The V/A ATPase from the thermophilic eubacterium Thermus thermophilus (Tth) is one of the best characterized rotary ATPases. The a-subunit is connected to the A3B3 stator in the V1 domain by two peripheral EG stalks which form a peripheral stator apparatus (A3B3E2G2a1). In addition, the dodecamer c ring composed of two transmembrane α-helices, the d-subunit and the DF shaft constitute the central rotor complex (D1F1d1c12), which rotates relative to the surrounding stator apparatus. The proton motive force generated by respiratory complexes drives proton translocation through a proton pathway made up of both the a-subunit and the c12 ring.

After refinements, 57.9 % of the particles corresponded to state1 and gave maps at a resolution of 5.0 Å, higher than those of state2 at 6.7 Å resolution and state3 at 7.5 Å, containing 15.2% and 6.3% of the particles, respectively. Local resolution analysis by Resmap22 for state1 showed a range of resolution from ~ 4 Å in the V1 region to ~ 5 Å in the Vo domain, indicating conformational heterogeneity within the complex. Local resolution of the hydrophobic region, especially of the c12 ring, was limited to ~ 6 Å due to conformational heterogeneity even within the most populated state1 structure. In order to improve resolution of the Vo domain, we employed the focused classification by using signal subtraction of hydrophilic region for state1, as described in Supplementary Figure 3. The improved map of state1 at 5.0 Å resolution allowed us to build a model of the whole complex. The inclined α-helices a-TM7 and a-TM8 are intimately associated with the c12 ring composed of 12 c-subunits, each with two transmembrane α-helices joined by a short loop on the cytoplasmic side. The tilted a-TM7 contains the conserved R563, corresponding to R735 in the yeast enzyme, which together with E63 in the c-subunit forms an essential feature of proton translocation. The density for a-TM7, where the R563 is located, is in close proximity to the center of an outer helix of the c-subunit. The cytoplasmic cavity provides direct access to the hydrophilic residues on a-TM7, reaching the Arg-Glu pair between a-TM7 and the outer helix of c-subunit, suggesting that this cavity corresponds to the cytoplasmic half channel. The periplasmic cavity in the center of micelle shell faces the helix bundle composed of a-TM1, a-TM2, and a-TM3, including a line of hydrophilic residues, and connects to the aqueous hole giving an access to the inclined helices.

>[3x]MIQGVIQKIAGPAVIAKGMLGARMYDICKVGEEGLVGEIIRLDGDTAFVQVYEDTSGLKVGEPVVSTGLPLAVELGPGMLNGIYDGIQRPLERIREKTGIYITRGVVVHALDREKKWAWTPMVKPGDEVRGGMVLGTVPEFGFTHKILVPPDVRGRVKEVKPAGEYTVEEPVVVLEDGTELKMYHTWPVRRARPVQRKLDPNTPFLTGMRILDVLFPVAMGGTAAIPGPFGSGKTVTQQSLAKWSNADVVVYVGCGERGNEMTDVLVEFPELTDPKTGGPLMHRTVLIANTSNMPVAAREASIYVGVTIAEYFRDQGFSVALMADSTSRWAEALREISSRLEEMPAEEGYPPYLAARLAAFYERAGKVITLGGEEGAVTIVGAVSPPGGDMSEPVTQSTLRIVGAFWRLDASLAFRRHFPAINWNGSYSLFTSALDPWYRENVAEDYPELRDAISELLQREAGLQEIVQLVGPDALQDAERLVIEVGRIIREDFLQQNAYHEVDAYCSMKKAYGIMKMILAFYKEAEAAIKRGVSIDEILQLPVLERIGRARYVSEEEFPAYFEEAMKEIQGAFKALA;>MDLLKKEYTGITYISGPLLFVENAKDLAYGAIVDIKDGTGRVRGGQVIEVSEEYAVIQVFEETTGLDLATTSVSLVEDVARLGVSKEMLGRRFNGIGKPIDGLPPITPEKRLPITGLPLNPVARRKPEQFIQTGISTIDVMNTLVRGQKLPIFSGSGLPANEIAAQIARQATVRPDLSGEGEKEEPFAVVFAAMGITQRELSYFIQEFERTGALSRSVLFLNKADDPTIERILTPRMALTVAEYLAFEHDYHVLVILTDMTNYCEALREIGAAREEIPGRRGYPGYMYTDLATIYERAGVVEGKKGSVTQIPILSMPDDDRTHPIPDLTGYITEGQIQLSRELHRKGIYPPIDPLPSLSRLMNNGVGKGKTREDHKQVSDQLYSAYANGVDIRKLVAIIGEDALTENDRRYLQFADAFERFFINQGQQNRSIEESLQIAWALLSMLPQGELKRISKDHIGKYYGQKLEEIWGAPQALD[3x];> MSQVSPTRMNLLQRRGQLRLAQKGVDLLKKKRDALVAEFFGLVREAMEARKALDQAAKEAYAALLLAQAFDGPEVVAGAALGVPPLEGVEAEVENVWGSKVPRLKATFPDGALLSPVGTPAYTLEASRAFRRYAEALIRVANTETRLKKIGEEIKKTTRRVNALEQVVIPGIRAQIRFIQQVLEQREREDTFRLKRIKGKIEAREAEEEGGRPNPQVEIGAGL;> MAVIADPETAQGFRLAGLEGYGASSAEEAQSLLETLVERGGYALVAVDEALLPDPERAVERLMRGRDLPVLLPIAGLKEAFQGHDVEGYMRELVRKTIGFDIKL;>MTGGLVLNAISRAGGAMGGLGLIKSLAEKEKQLLERLEAAKKEAEERVKRAEAEAKALLEEAEAKAKALEAQYRERERAETEALLARYRERAEAEAKAVREKAMARLDEAVALVLKEVLP[2x];>[2x]MSKLEAILSQEVEAEIQALLQEAEAKAEAVKREAEEKAKALLQARERALEAQYRAALRRAESAGELLVATARTQARGEVLEEVRRRVREALEALPQKPEWPEVVRKLALEALEALPGAKALVANPEDLPHLEAMARERGVELQAEPALRLGVRAVGAEGKTQVENSLLARMDRAWDAMSSKVAQALWG;> MADDFAYLNARVRVRRGTLLKESFFQEALDLSFADFLRLLSETVYGGELAGQGLPDVDRAVLRTQAKLVGDLPRLVTGEAREAVRLLLLRNDLHNLQALLRAKATGRPFEEVLLLPGTLREEVWRQAYEAQDPAGMAQVLAVPGHPLARALRAVLRETQDLARVEALLAKRFFEDVAKAAKGLDQPALRDYLALEVDAENLRTAFKLQGSGLAPDAFFLKGGRFVDRVRFARLMEGDYAVLDELSGTPFSGLSGVRDLKALERGLRCVLLKEAKKGVQDPLGVGLVLAYVKEREWEAVRLRLLARRAYFGLPRAQVEEEVVCP;> MIAPMEKLVLAGPKGRAKELLQSLQQAGVVHLETLRPEALSAYQLSPEERAELRRWEAVSAGAEHTLSLLGLEAEPARPFPEGLEAAEKALSPIQAHAEGLTRQKQELEEELALAQAYLEPLERLAALAHGLDKSPFLRVIPFLLTEKELPLVEEALRKALEDRYLLAHEAYAGGVAALVVVHRKEVDQAKAALSRAGVAELRLPGALGELPLSEAARRLKERAEAAPRELSEVRQHLAKLARESASTLQSLWTRAQDEVARLKALEELASGRFGFALLGYVPVKAKPKVEEALARHKESVVYAFEPVDEHHEADRIPVVLDNPPWAKPFELLVSFLNTPKYGTFDPTPVVPVFFPFWFGMIVGDIGYALLFYLVGRWLSGYVKRNEPLVIDLFALKLKPQVIGKLVHILNWMVFWTVVWGVIYGEFFGTFLEHLGVFGTPEHPGLIPILIHRIDTAKTANLLILLSVAFGVVLVFFGLALRAYLGLKHRHMAHFWEGVGYLGGLVGVLALAASYLGNLQAGWLQGLMYLGFGVFLLAVLMSRIWLMIPEIFTQAGHILSHIRIYAVGAAGGILAGLLTDVGFALAERLGLLGVLLGLLVAGVLHLLILLLTTLGHMLQPIRLLWVEFFTKFGFYEENGRPYRPFKSVREAQ;>MKKLLVTVLLAVFGALAFAAEEAAASGGLDRGLIAVGMGLAVGLAALGTGVAQARIGAAGVGAIAEDRSNFGTALIFLLLPETLVIFGLLIAFILNGRL[12x]>RSVRVLVDMDGVLADFEAGLLRGFRRRFPEEPHVPLEQRRGFLAREQYRALRPDLADKVASVYEAPGFFLDLEPIPGALDAVREMNDLPDTQVFICTSPLLKYHHCVGEKYRWVEQHLGPQFVERIILTRDKTVVLGD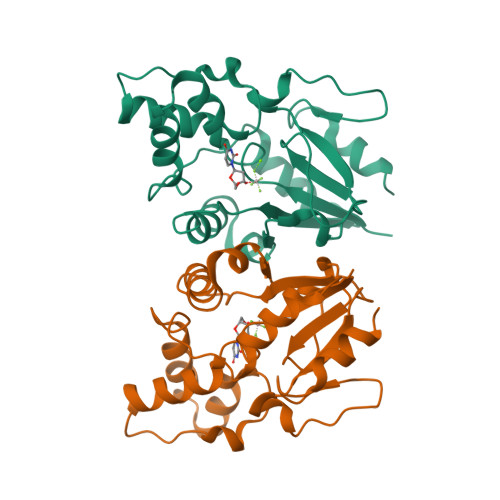LLIDDKDTVRGQEETPSWEHILFTCCHNRHLVLPPTRRRLLSWSDNWREILDSKR[2x]The type VI secretion system (T6SS) delivers enzymatic effectors into target cells to destroy them. Here, we report the identification and characterization of a Tle3 phospholipase effector and its cognate immunity protein Tli3—an outer membrane lipoprotein from adherent-invasive Escherichia coli (AIEC). Enzymatic assays demonstrate that purified Tle3AIEC has a phospholipase A1, and not A2, activity and that its toxicity is neutralized by the cognate immunity protein Tli3AIEC. Tli3AIEC binds Tle3 in a 1:1 stoichiometric ratio.

The Tle3AIEC-Tli3AIEC complex structure could not be solved by SeMet phasing, but only by molecular replacement when using an AlphaFold2 prediction model. Finally, the 8 complexes exhibited a reasonable geometry for a 3.6 Å resolution with R and Rfree factors of 23.4% and 26.8%, respectively. Tle3AIEC shares the classical core of an α/β-hydrolase fold, with a β-sheet of six parallel β-strands in the order β2β1β3β4β5β6. In Tle3AIEC, the catalytic serine was identified in a short loop between a β–strand and a α–helix, with the sequence SHSQG at position 265. The Ser265 hydroxyl moiety is implicated in a hydrogen bound with the Ne2 atom of His574 which is, in turn, hydrogen-bound by its Nd1 atom to the Asp377 carboxyl group, forming the catalytic triad. A cation, probably Ca2+, is observed at bonding distance from three acidic side chains from Asp444, Asp484 and Asp573 and the C=O group of Asp377. Notably, Asp377 C=O group participates in the binding of the Ca2+ cation, whose function might be to stabilize the catalytic triad geometry. The catalytic triad is located at the bottom of a crevice ~30-Å deep and ~20 × 15 Å. The core of Tli3AIEC is assembled in three stacked β-sheets of 4, 3 and 4 β-strands, respectively, with topology of β1β2β3β4, β6β7β8, β5β10β11β12. The β6-β7 Tli3AIEC loop inserts deeply in the Tle3AIEC substrate-binding crevice, without reaching catalytic Ser265, however.

>[8x]MSTNKSEPTRKVDVHLTDNGTPFAYSMTSHKNVKVRAEVQPPLQLPGLIIFVHGVNSEGEWYDYAERSLCAGLNQRLGLEGEHGLKENNYEGGFFVNSDKSEGGWEHTYEIEGSQKKWVSGPRKITKGGDGRSPVIRFYWGYRAADNETDTYAIPLKNKKGDNYYDLPPESRKAKGPWFWGGGPFQNGCNQLVSLWSKTGFNNNPSLLGVPLPFSTQVLNGERDRLLSDAPPRHYYAHAAGRLAKLIKTIRNQHPEDTVTVLSHSQGTMIALAAAAIEAPDALFVMNSPYALENEPTTYISYPIKEIISRKARSATFADIVKKVAENKTRLKQQGCDNLLAGMSSDGNSWIPEGKTHNGLPERDNHGTTWIYCNPHDRVMGSSPLRSIGWQGLPDTKDGTPHTLFKQAGDTLYVRILGRNTPCGGTPTAQTHFSNLGDGKPFWDSTTTLLQRATWPDPDSGQTLTINAPQVPEPLTAEELKNFDQDYARDEKQSGGAGYAYGQINPETKKPVDTDYRYYISLYGYFDRKMVPKKDSGYYQSGPGSKEDRVKYEKQSQEEMLEEVRTYVQRPTDHSTLPSDERFMSRVVAYDLPIGYCWHSWDKAGLEELRRQADWLESDDYYFSGKLTVPPIPPAIKQDVAEDAEQRKAEEKARLRNV;>[8x]MLKEWMIFTCSLLTLAGASLPLSGCISRGQESISEGAAFGAGILREPGATKKADTKDLNVPPPVYGPPQVIFRIDDNRYFTLENYTHCENGQTFYNNKAKNIHVKILDASGYLFKGRLFWLSTRDDFLAFPATLNTRHASCMGSNKGCMNAVIVTTDGGKRRSGVPYGSYTQNPTGATRDYDMLVMNDGFYLLRYRGGQGRFSPVILRWILSTEDSSGVVRSEDAYELFRPGEEVPSTGFYKIDLSRFYPKNNVMEMQCDRTLEPVQPSESKIQ> VNTITFDVGNATINKYATFMESLRNEAKDPTLKCYGIPMLPDSNLTPKYVLVKLQDASSKTITLMLRRNNLYVMGYSDLYNGKCRYHIFNDISSTESTDVENTLCPNSNSREKKAINYNSQYSTLQNKAGVSSRSQVQLGIQILNSDIGKISGVSTFTDKTEAEFLLVAIQMVSEAARFKYIENQVKTNFNRAFNPNPKVLSLEENWGKISLAIHNAKNGALTSPLELKNADDTKWIVLRVDEIKPDMGLLNYV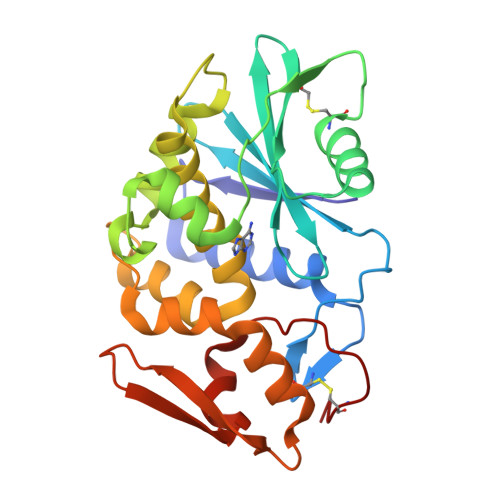SGTCQTT> MGRIEVVNVSHIFHRGTPLEKKALENVSLVINEGECLLVAGNTGSGKSTLLQIVAGLIEPTSGDVLYDGERKKGYEIRRNIGIAFQYPEDQFFAERVFDEVAFAVKNFYPDRDPVPLVKKAMEFVGLDFDSFK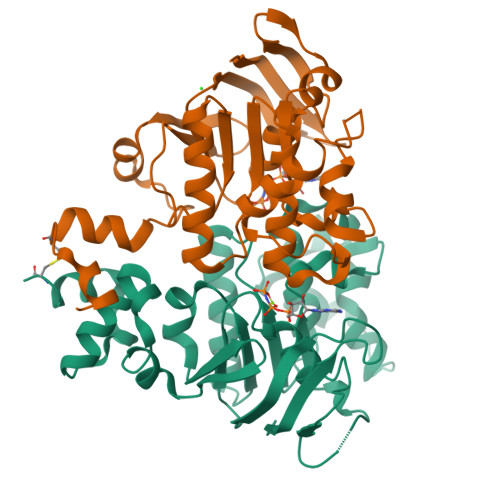DRVPFFLSGGEKRRVAIASVIVHEPDILILDEPLVGLDREGKTDLLRIVEKWKTLGKTVILISHDIETVINHVDRVVVLEKGKKVFDGTRMEFLEKYDPRFFTSKMLVMRRLVLKGEDPFSMSDDELLERVCNS;> GSGGSHMGSGRIELNSVSFRYNGDYVLKDVNAEFETGKIYVVVGKNGSGKTTLLKILAGLLAAAGEIFLDGSPADPFLLRKNVGYVFQNPSSQIIGATVEEDVAFSLEIMGLDESEMRKRIKKVLELVGLSGLAAADPLNLSGGQKQRLAIASMLARDTRFLALDEPVSMLDPPSQREIFQVLESLKNEGKGIILVTHELEYLDDMDFILHISNGTIDFCGSWEEFVEREFDDVEIPFKWKLWKKCGKINLWEDRYENSGNQRRRDTV Oxidation of SLA is catalyzed by SLA dehydrogenases belonging to the aldehyde dehydrogenase superfamily. SLA dehydrogenases (annotated as GabD or SlaB) belong to the sequence-based protein family PF00171 within the Pfam database, which are members of the aldehyde dehydrogenase superfamily. We report that SLA dehydrogenase RlGabD from the sulfoglycolytic bacterium Rhizobium leguminsarum SRDI565 can use both NAD+ and NADP+ as cofactor to oxidize SLA, and indicatively operates through a rapid equilibrium ordered mechanism. SLADH enzymes catalyze the oxidation of SLA to SL, the final step of sulfoglycolytic pathways that lead to excretion of SL,4 and the second step in the oxidation of DHPS to SL in Desulfovibrio sp.,5 which activates this substrate for sulfur–carbon bond scission in the DHPS degradation pathway to produce sulfite and pyruvate.

Thus, cryo-EM grids were optimised and prepared with 1 mg mL−1RlGabD pre-incubated with 2 mM NADH. The RlGabD tetramer assembles as a pair of dimers. Each L-shaped protomer comprises an α/β N-terminal cofactor binding domain [residues 8–133, 153–263], an α/β catalytic domain containing the conserved Cys-Glu dyad [residues 264–476], and a smaller, anti-parallel β-sheet oligomerization domain [residues 134–152, 477–489], which interacts with two other subunits. The RlGabD dimer is formed through domain swapping interactions of the three-stranded oligomerization domain of subunit A with the catalytic domain of partner subunit (B) forming a ten-stranded β-sheet. However, this still allowed NADH to be modelled with confidence, and showed that NADH is bound in an extended mode, as seen in E. coli SSADH GabD,23 with the nicotinamide group protruding into the active site located in the cleft between the two major domains. The nicotinamide ring sits in close vicinity to the catalytic dyad, and the adenine ring occupies a hydrophobic pocket lined by Ala 219, Leu224, Val243, Trp246, and Leu247. The RlGabD·NADH complex displays the catalytically-relevant ‘in’ conformation with the nicotinamide ring pointing into the active site, and C4 of nicotinamide approx. 6.7 Å from catalytic Cys295. Thus, we propose that Cys295 is the catalytic nucleophile, Glu261 is the general base, and the oxyanion hole is formed from Asn163 and the backbone NH of Cys295.

>[4x]MTERRTLALKDPALLTDKAFVAGAWIGAPDGKSIAVTDPFDGALIANVPDLGQAVVAQAIDAAAEAQKLWERRTAKERAQVLKRWYDLIVENADDLALILTTEQGKPLAEARGEVVSNAAYLEWFAEEAKRIDGDIIPGPNAGQRIMVLKQPVGVCAAITPWNFPNGMITRKAGPALAAGCSMILKPASQTPLSALALAVLAERAGVPKGVFSVVTGEAKPIGLEFCHNPRIAKITFTGSTGVGRWLMKEAAGGIKRLSLELGGNAPFIVFDDADLDAAVEGAMISKFRNAGQTCVCANRIYVQESVAAAFTERLLAKVSGLSLGRGTDAGVSQGPLIDEKAVAKMEEHIADAMANGGTVLTGGKRSVLGGTFFEPTVVTGVTQTMKVAKEETFAPLAPIISFKHENDVIAMANDSEFGLASYFYAKDMARIWRVAEALEAGMVGVNTGMIANEMAPFGGIKQSGTGREGSKYGIEGFLELKYVALGGMLEHHHHHH> MKPYQRQFIEFALNKQVLKFGEFTLKSGRKSPYFFNAGLFNTGRDLALLGRFYAEALVDSGIEFDLLFGPAYKGIPIATTTAVALAEHHDKDLPYCFNRKAAKDHGEGGSLVGSALQGRVMLVDDVITAGTAIRESMEIIQAHGATLAGVLISLDRQERGRGEISAIQEVERDYGCKVISIITLKDLIAYLEEKPDMAEHLAAV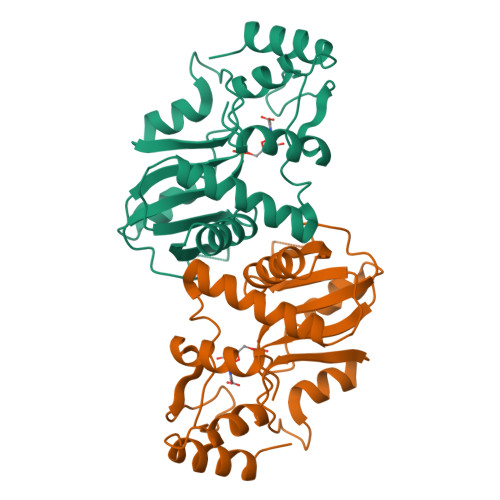RAYREEFGV>RCLFVCRHGERMDVVFGKYWLSQCFDAKGRYIRTNLNMPHSLPQRSGGFRDYEKDAPITVFGCMQARLVGEALLESNTIIDHVYCSPSLRCVQTAHNILKGLQQENHLKIRVEPGLFE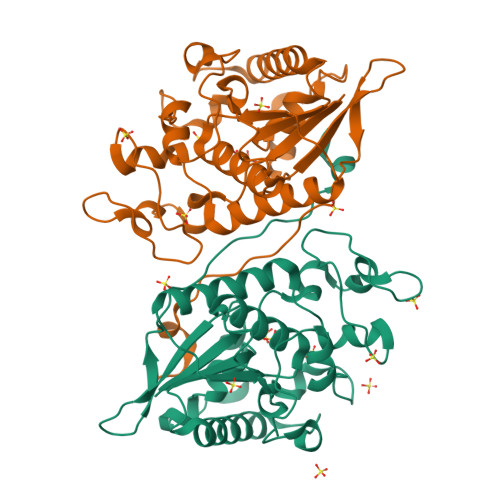WTKWVAGSTLPAWIPPSELAAANLSVDTTYRPHIPISKLVVSESYDTYISRSFQVTKEIISECKSKGNNILIVAHASSLEACTCQLQGLSPQNSKDFVQMVRKIPYLGFCSCEELGETGIWQLTDPPILPLTHGPTGGFNWRETLLQE[2x]> IINGEDCSPHSQPWQAALVMENELFCSGVLVHPQWVLSAAHCFQNSYTIGLGLHSLEADQEPGSQMVEASLSVRHPEYNRPLLANDLMLIKLDESVSESDTIRSISIASQCPTAGNSCLVSGWGLLANGRMPTVLQCVNVSVVSEEVCSKLYDPLYHPSMFCAGGGQDQKDSCNGDSGGPLICNGYL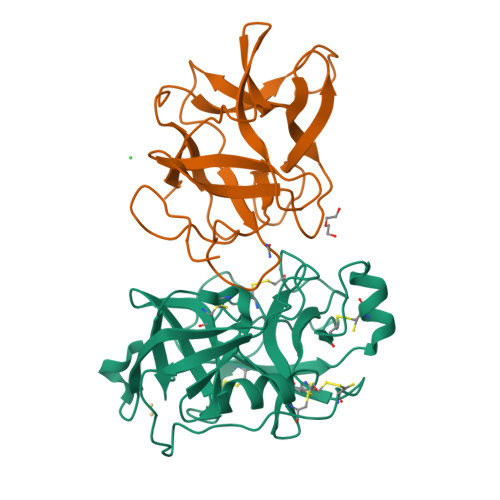QGLVSFGKAPCGQVGVPGVYTNLCKFTEWIEKTVQA;> GSSVVVDTNGQPVSNGADAYYLVPVSHGHAGLALAKIGNEAEPRAVVLDPHHRPGLPVRFESPLRINIIKESYFLNIKFGPSSSDSGVWDVIQQDPIGLAVKVTDTKSLLGPFKVEKEGEGYKIVYYPERGQTGLDIGLVHRNDKYYLAVKDGEPCVFKIRKAT> GVQLTAAQELMIQQLVAAQLQCNKRSFSDQPKVTPWPLGADPASGSASQQRFAHFTELAIISVQEIVDFAKQVPGFLQLGREDQIALLKASTIEIMLLETARRYNHETECITFLKDFTYSKDDFHRAGLQVEFINPIFEFSRAMRRLGLDDAEYALLIAINIFSADRPNVQEPGRVEALQQPYVEALLSYTRIKRPQDQLRFPRMLMKLVSLRTLSSVHSEQVFALRLQDKKLPP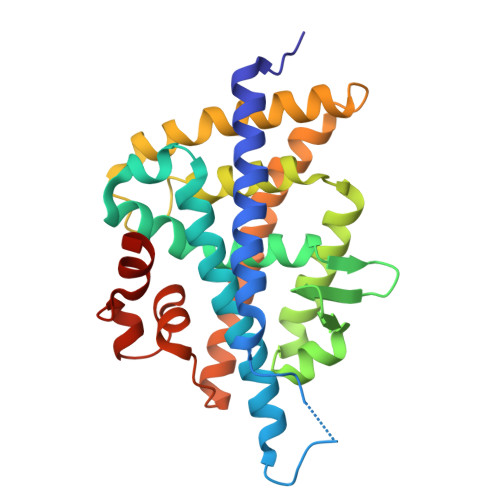LLSEIWDVHEGSGSGSHKILHRLLQDSSS> MKVLWAALLVTFLAGCQAKVEQAVETEPEPELRQQTEWQSGQRWELALGRFWDYLRWVQTLSEQVQEELLSSQVTQELR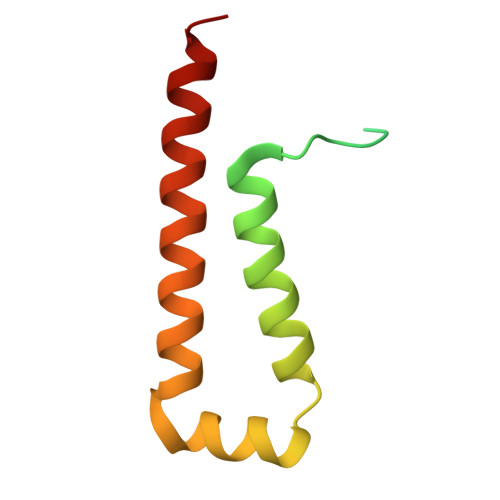ALMDETMKELKAYKSELEEQL N-(4-methylpyridin-3-yl)acetamide | C8 H10 N2 O | 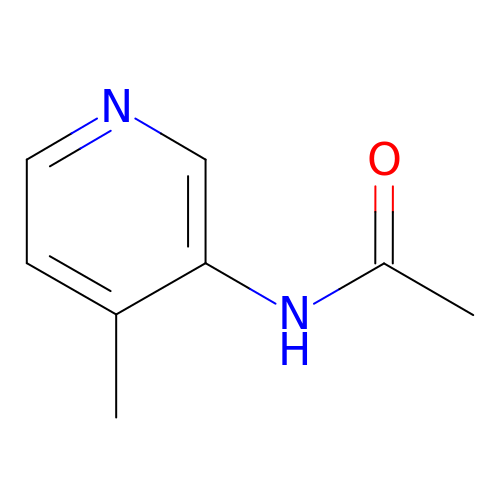WRPYDRDMRXJIJA-UHFFFAOYSA-N> SNAMTTILPNLPTGQKVGIAFSGGLDTSAALLWMRQKGAVPYAYTANLGQPDEPDYDEIPRRAMQYGAEAARLVDCRAQLVAEGIAALQAGAFHISTAGLTYFNTTPIGRAVTGTMLVAAMKEDGVNIWGDGSTFKGNDIERFYRYGLLTNPDLKIYKPWLDQTFIDELGGRAEMSEYMRQAGFDYKMSAEKAYSTDSNMLGATHEAKDLELLSAGIRIVQPIMGVAFWQDSVQIKAEEVTVRFEEGQPVALNGVEYADPVELLLEANRIGGRHGLGMSDQIENRIIEAKSRGIYEAPGLALLFIAYERLVTGIHNEDTIEQYRENGRKLGRLLYQGRWFDPQAIMLRETAQRWVARAITGEVTLELRRGNDYSLLNTESANLTYAPERLSMEKVENAPFTPADRIGQLTMRNLDIVDTREKLFTYVKTG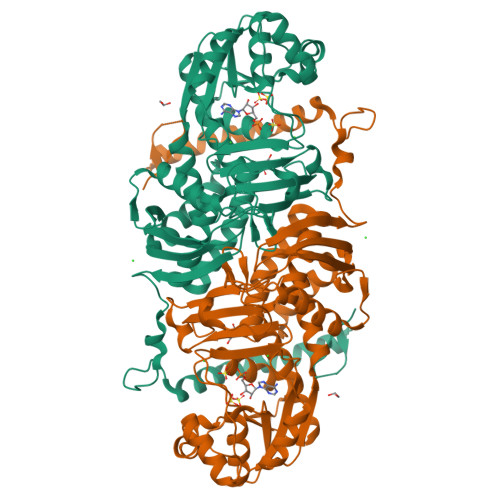LLAPSAGSALPQIKDGKK>[4x]MAKKTSSKGKLPPGPTPLPFIGNYLQLNTEQMYNSLMKISERYGPVFTIHLGPRRVVVLCGHDAVREALVDQAEEFSGRGEQATFDWVFKGYGVVFSNGERAKQLRRFSIATLRDFGVGKRGIEERIQEEAGFLIDALRGTGGANIDPTFFLSRTVSNVISSIVFGDRFDYKDKEFL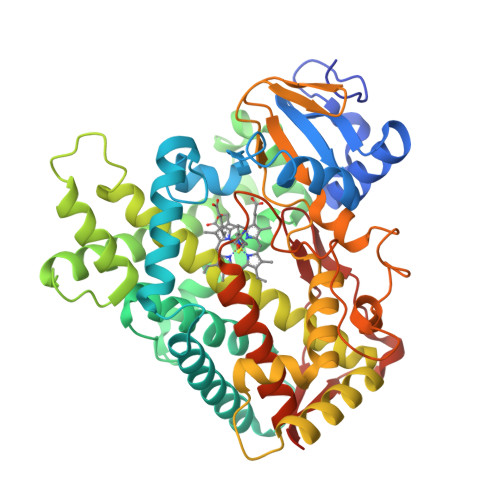SLLRMMLGSFQFTSTSTGQLYEMFSSVMKHLPGPQQQAFQLLQGLEDFIAKKVEHNQRTLDPNSPRDFIDSFLIRMQEEEKNPNTEFYLKNLVMTTLNLFFAGTETVSTTLRYGFLLLMKHPEVEAKVHEEIDRVIGKNRQPKFEDRAKMPYMEAVIHEIQRFGDVIPMGLARRVKKDTKFRDFFLPKGTEVYPMLGSVLRDPSFFSNPQDFNPQHFLNEKGQFKKSDAFVPFSIGKRNCFGEGLARMELFLFFTTVMQNFRLKSSQSPKDIDVSPKHVGFATIPRNYTMSFLPRHHHH>[4x]AQYEDGKQYTTLEKPVAGAPQVLAFFSFFCPHCYQ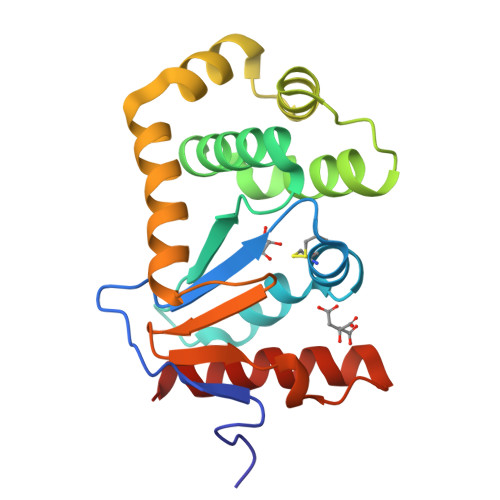FAEVLHISDNVKKKLPEGVKMTAYHVNFMGGDLGKDLTQAWAVAMALGVEDKVTVPLFEGVQKTQTIRSASDIRDVFINAGIKGEEYDAAWNSFVVKSLVAQQEKAAADVQLRGVPAMFVNGKYQLNPQGMDTSNMDVFVQQYADTVKYLSEKK[(5S,6E,8S,9S,12R,13E,15E)-21-chloranyl-12,20-dimethoxy-6,8,16-trimethyl-5-oxidanyl-3,11-bis(oxidanylidene)-2-azabicyclo[16.3.1]docosa-1(21),6,13,15,18(22),19-hexaen-9-yl] 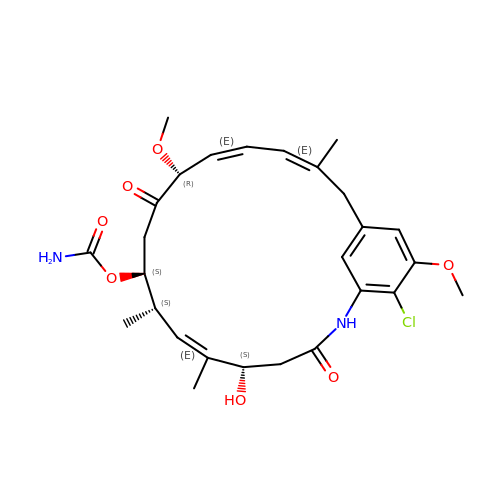carbamate | C27 H35 Cl N2 O7 | ZVEKPDFJWUKDJA-RWGYLTEZSA-N> SYFQSNVVIA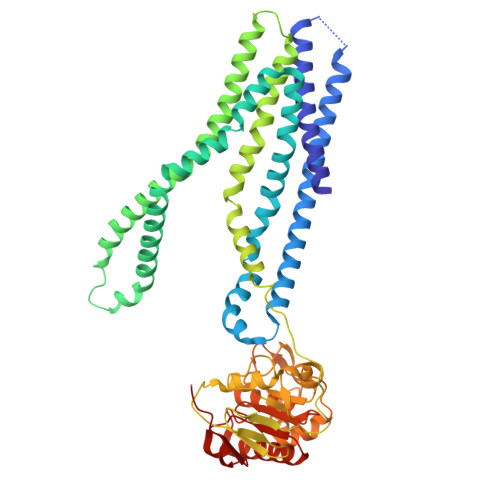GCTIASAVVLAHIVAGIITNPATALGGETDWAPGLVALAVLWSVRVVAQWFQGRLSQRGATAVIGELSRQVLSSVTTSSPRRLAADRDSAAAVVTRGLDGLRPYFTGYLPAVVLAGILTPAALVVMAAYDWQAAAIVVIALPLIPIFMVLIGLLTAERSAAALTAMTTLQGRMLDLIAGIPTLRAVGRAGGSVQRIAELSASHRRSTMATLRISFLSALVLELLATLGVALVAVSVGLRLVFGDMTLAAGLTALLLAPEVFWPLRRVGAAFHAAQDGKTAAEQALRLCAEPHPPTGHEVVPAGAPVIEVPALKAVMEPGRVTVLTGPNGVGKSTLLQAILGLQESPCGPILVAGVEVGALDRSAWWGRLAWMPHRPVLVPGTVRENLELLGPVPGLDEVCRSVGFDEVLGELPDGSETPLGRGGVGLSLGQRQRLGLVRALGAPADVLLLDEPTAHLDGALEDRVLAAIVARARAGATVVMVGHRAPVLAAADHVVTMESSLVAP>[4x]MAGPLSGLRVVELAGIGPGPHAAMILGDLGADVVRIDRPSSVDGISRDAMLRNRRIVTADLKSDQGLELALKLIAKADVLIEGYRPGVTERLGLGPEECAKVNDRLIYARMTGWGQTGPRSQQAGHDINYISLNGILHAIGRGDERPVPPLNLVGDFGGGSMFLLVGILAALWERQSSGKGQVVDAAMVDGSSVLIQMMWAMRATGMWTDTRGANMLDGGAPYYDTYECAD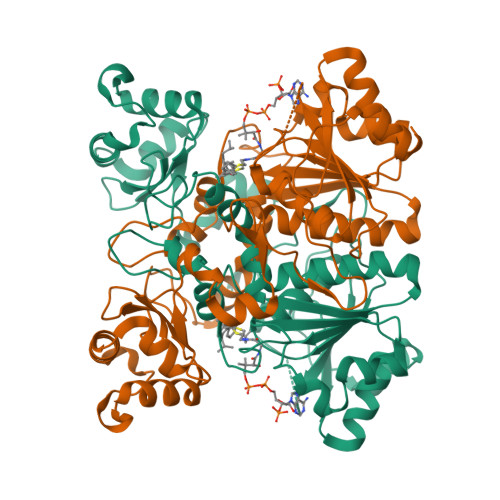GRYVAVGAIEPQFYAAMLAGLGLDAAELPPQNDRARWPELRALLTEAFASHDRDHWGAVFANSDACVTPVLAFGEVHNEPHIIERNTFYEANGGWQPMPAPRFSRTASSQPRPPAATIDIEAVLTDWDG> GAMGASVRPNMSRICLIPSSELQTKLDKKLGAGAFGTVFAGIYYPKRAKNVKIPVAIKVFQTDQSQTDEMLEEATNMFRLRHDNLLKIIGFCMHDDGLKIVTIYRPLGNLQNFLKLHKENLGAREQVLYCYQIASGMQYLEKQRVVHRDLATRNVLVKKFNHVEITDFGLSKILKHDADSITIKSGKVAIKWLAIEIFSKHCYTHASDVWAFGVTCW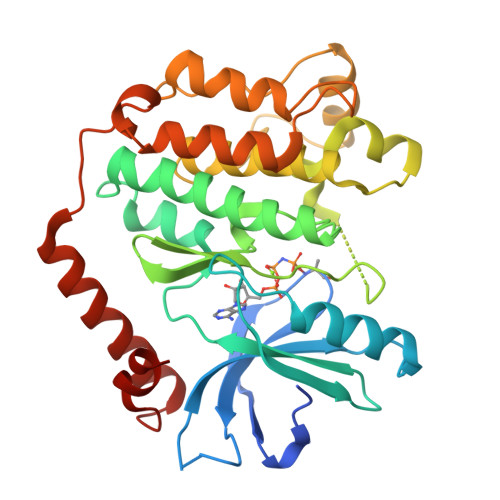EIITFGQSPYQGMSTDSIHNFLKDGNRLSQPPNCSQDLYQELLRCWMADPKSRPGFEILYERFKEFCKVPQLFLENSNKISESDLSAEERFQTERIREMFDGNIDPQMYFDQG3-({6-chloro-3-[3-(4-chloro-3,5-dimethylphenoxy)propyl]-7-(1,3,5-trimethyl-1H-pyrazol-4-yl)-1H-indole-2-carbonyl}amino)benzoic 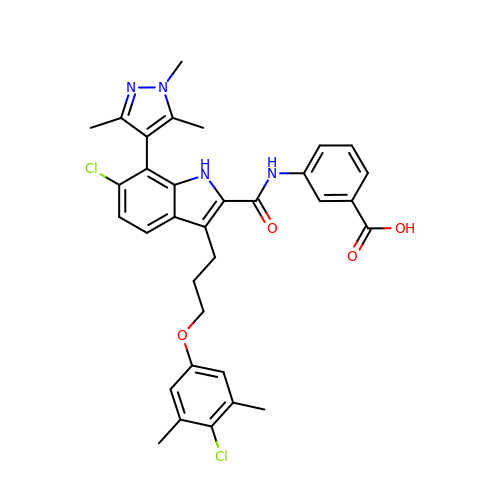acid | C33 H32 Cl2 N4 O4 | ODMWLLDLJAHWIY-UHFFFAOYSA-N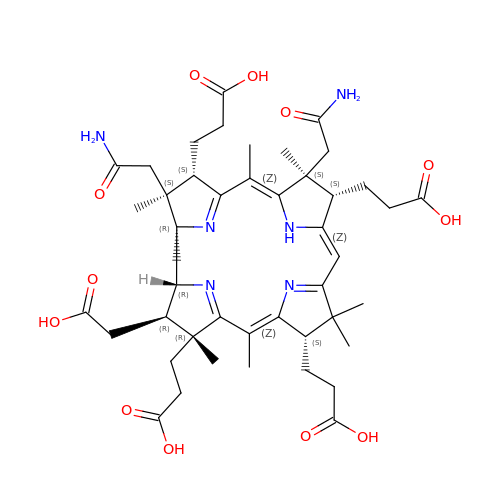Hydrogenobyrinic acid a,c-diamide | C45 H62 N6 O12 | ZGGWTIPDUOTHRA-NREUJTCUSA-N>GSHMAPGFTISFVNKTIIVTGGNRGIGLAFTRAVAAAGANVAVIYRSAADAVEVTEKVGKEFGVKTKAYQCDVSNTDIVTKTIQQIDADLGPISGLIANAGVSVVKPATELTHED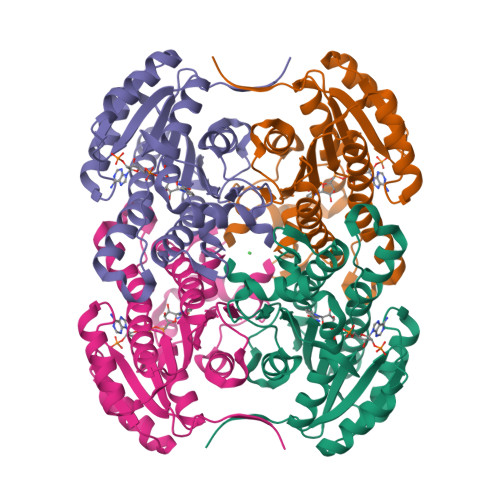FAFVYDVNVFGVFNTCRAVAKLWLQKQQKGSIVVTSSMSSQIINQSSLNGSLTQVFYNSSKAACSNLVKGLAAEWASAGIRVNALSPGYVNTDQTAHMDKKIRDHQASNIPLNRFAQPEEMTGQAILLLSDHATYMTGGEYFIDGGQLIW[12x]>SNAMHSPQISPPIAPSTPLLAGWRSAGKAPEAAIRGEAVSLQPLDAPRHGAALFRLFAGDDSHWEHLPYGPFEDEDAFITWLALTVAQSDTALYVVCAKDSDQALGFLGYRQMVQAHGAIEIGHVNFSPALRRTRLATEAVFLLLKTAFELGYRRCEWRCDSRNAASAAAARRFGFQFEGTLRQAM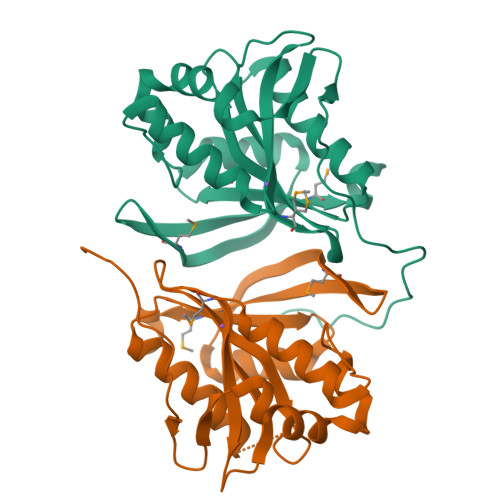VVKRRNRDTHVFSMLDGEWDALK[2x]(4S)-4-[2,4-difluoro-5-({[1-(trifluoromethyl)cyclopropyl]amino}methyl)phenyl]-4-methyl-5,6-dihydro-4H-1,3-thiazin-2-amine 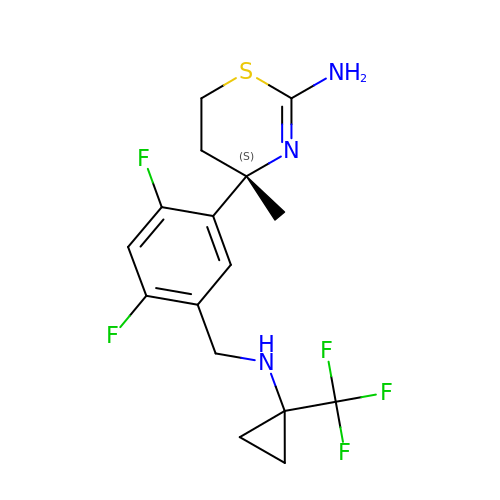| C16 H18 F5 N3 S | XKONRMXLBXCJAM-AWEZNQCLSA-N> GSEFSAKDERAREILRGFKLNWMNLRDAETGKILWQGTEDLSVPGVEHEARVPKKILKCKAVSRELNFSSTEQMEKFRLEQKVYFKGQCLEEWFFEFGFVIPNSTNTWQSLIEAAPESQMMPASVLTGNVIIETK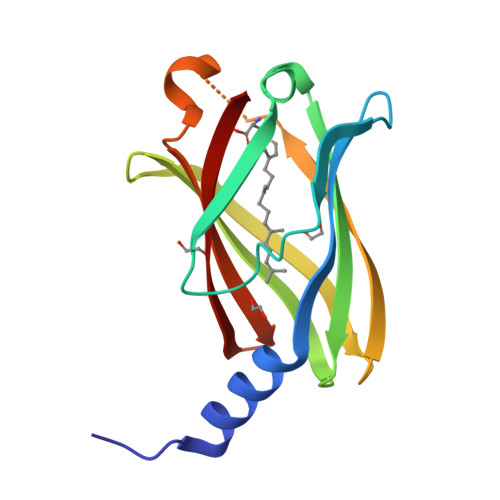FFDDDLLVSTSRVRLFYV>MKKIITLFGACALAFSMANADVNLY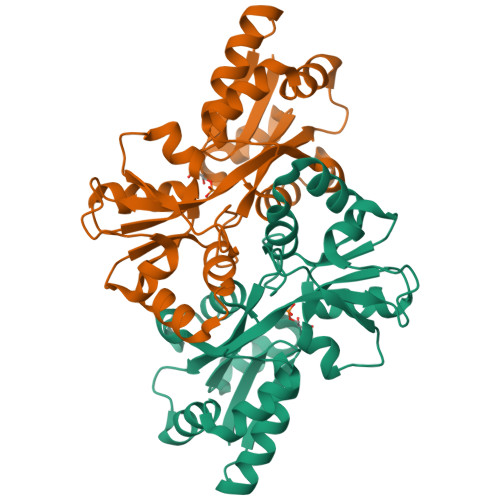GPGGPHTALKDIANKYSEKTGVKVNVNFGPQATWFEKAKKDADILFGASDQSALAIASDFGKDFNVSKIKPLYFREAIILTQKGNPLKIKGLKDLANKKVRIVVPEGAGKSNTSGTGVWEDMIGRTQDIKTIQNFRNNIVAFVPNSGSARKLFAQDQADAWITWIDWSKSNPDIGTAVAIEKDLVVYRTFNVIAKEGASKETQDFIAYLSSKEAKEIFKKYGWREH[4x]>GNDEVENLGNNVPGEQAVLTIKLKGDGDNQAQSRAAGPATDTEDAVINNYLVFLFREGGALDCAPYEGSSNAAATITTGTTAAKKAYVVANTGALAGGLFATVKTETDLLAVTGSLMDNTDNASTQTKTNLWMSGESEVKFNGGTNAQVTVSLSFVAAKIQLIVKDNRKNMTGGTITITDDAAVLLFAGKKGRFFGSAAEKVTQNEFYTGFNQYTGAFDSGVTTSTALSDAVSPGDFTINAGSTVFNHFYTFGNDGTTQPTILAI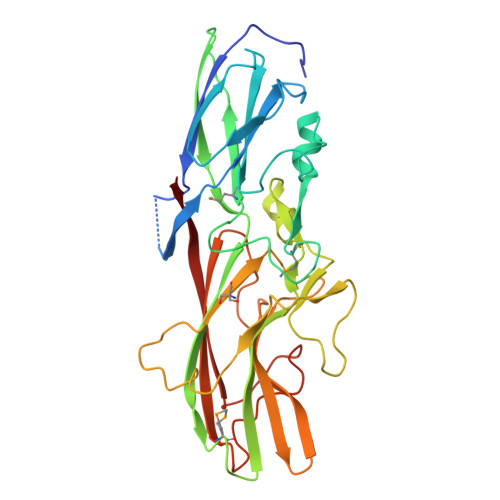KSTKTVGGTSSPIFYPILFTNTDARHTIEPGKSYTVTVTLNGDVAAGGGGGTTDPEEPVVSSSIEVTVTAAQWVTQPVDKEFN[2x]(2~{S},3~{S})-2-acetamido-~{N}-(3-bromanylprop-2-ynyl)-3-methyl-pentanamide | C11 H17 Br N2 O2 | 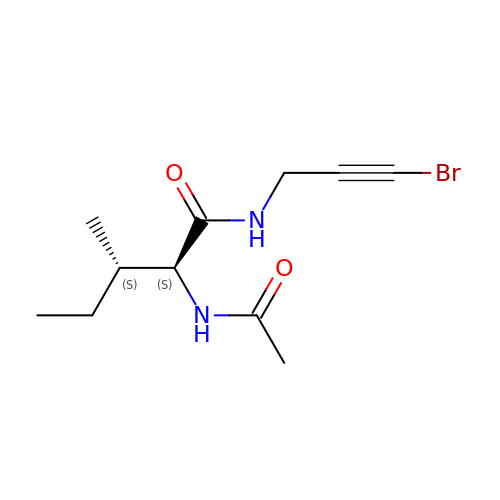RXUWJGHXIHPACB-WPRPVWTQSA-N> MKTMAKTQ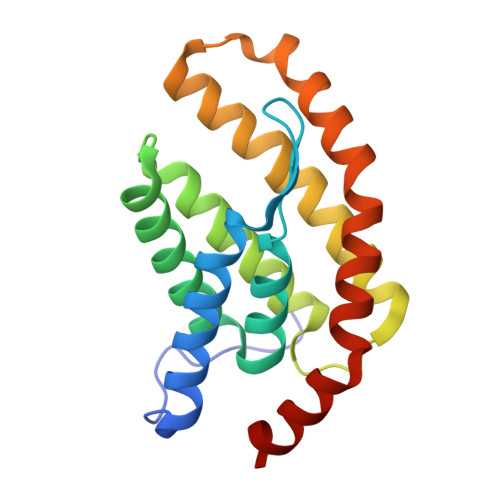LPKLDTLSMVTMGVLMALQLVISRFSVGNNFIKVSFTFLIVALIAKWFGPWWGMLTAAVVDVIGTLMTGGPFFIGFTVSAVLGSLIYAVFLYRQPVSWWRVIGASVLIALLVNTLLNTLWVTIMYQTPFWSLLPVRALKELIVTPVQIVLVYLLLKSQVIQMIQARLNK> MPVITVNTNVAEKSIPVFFQAALTNMMTKALQKPKEVMFVDLRSGANIMMGGDRNPCVFATVECIGRLNP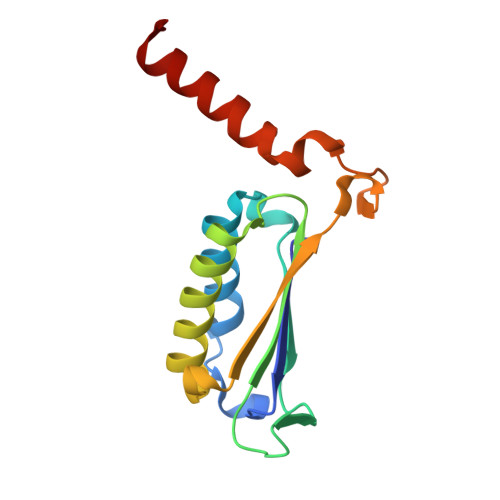TSNLAMARDMEDMFIEHLNVRRERIVIRFIPVPALFCSFNGALHDVSIERDEDIISQAIAEYLAAHAA> SMPKTISVRVTTMDAELEFAIQPNTTGKQLFDQVVKTIGLREVWFFGLQYQDTKGFSTWLKLNKKVTAQDVRKESPLLFKFRAKFYPEDVSEELIQDITQRLFFLQVKEGILN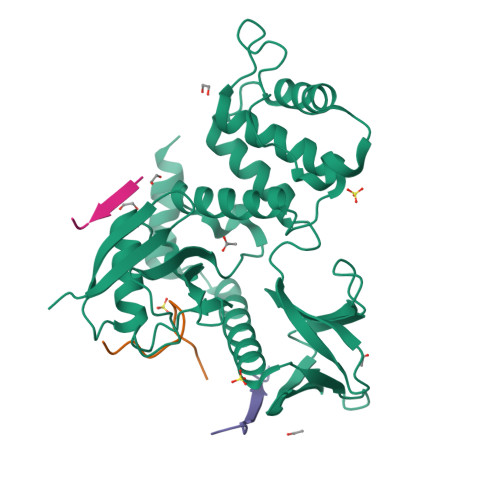DDIYCPPETAVLLASYAVQSKYGDFNKEVHKSGYLAGDKLLPQRVLEQHKLNKDQWEERIQVWHEEHRGMLREDAVLEYLKIAQDLEMYGVNYFSIKNKKGSELWLGVDALGLNIYEQNDRLTPKIGFPWSEIRNISFNDKKFVIKPIDKKAPDFVFYAPRLRINKRILALCMGNHELYMRRRKPDTIEVQQMKAQAREEKHQKQMERAMLENEKKKREMAEKEKEKIEREKEE;> EDGGSWKYPDAFELSG;> EDGGSSWEYIWTLPSG;> AAAAAG>[2x]MKVQYSFEREFEELMSDLLSKYGYEMFQMDGLGDQLDVVKFTEDFVRRGIIESTIDANANVRVTNISTYFIEISKPHTYLYSLYRIWQKMKEMFGKGVADEFVEAQINGAVYLHDRHHAALMPYCFAYTLKPIVEKGLPFIKTIKSEPAKHLSTFIQHVIQFVMFASNQSSGAVGLPDFFVWMWYFVKKDLKEGIIPRDKLDWYIEQHFQILTYSLNQPIRTTQSPYTNFTYLDRNYIKAIFEGERYPDGSLITDHVEDIIALQKHYWEWVSRERERQMFTFPVLTASLLYKDGKFLDEDSARFINKINMKWQDTNWYISDSIDAVASCCRLTSSTQTLKKFSLSSEEEEKLKGRMNSIGGSDLNIGSFKVITVNLPRIALESGGDREKYLQILRHRVQLIKKALAAVREIIKERISEGLLPLYENGLMLLNRQYGTIGVTGVWESASIMGLTTEDIDGLKYTEEGEVFVDNVLDTIREEAEKGYHEYGFTFNIEQVPAEKAAVTLAQKDRFLFGEKQPFEIYSNQWVPLMANTDVLNRIRYSGKWDKKVSGGAILHINLGESFKTEEESFNMVKMIADMGVMYFAFNTKISVCEDGHAFYGERCPVCGKAKVDEYMRIVGYLVPVSAFNKERREIEYPRRQFYDSLTIRR

Ribonucleotide reductases (RNRs) are highly important enzymes for all life, as they are solely responsible for the first committed step in the synthesis of the deoxyribonucleoside triphosphate (dNTP) building blocks of DNA. Class III RNRs, strictly anaerobic, generate on a separate activating enzyme NrdG the same type of 5’-dAdo radical through homolytic cleavage of a C-S bond in S-adenosylmethionine, with the participation of a [4Fe-4S] cluster. Here we present the crystal structure of a second class III RNR from Thermotoga maritima (tmNrdD), which, as purified and crystallized, surprisingly does not display such a cysteine, possessing an isoleucine (Ile) in its place. Nevertheless tmNrdD binds a substrate and its allosteric effector in productive conformations as expected from previous structures of RNRs of all three classes, and it is enzymatically active.

The native structure was solved from crystals obtained under three different conditions, one with the buffer molecule citrate bound in the active site, another with MES and a third with glycerol. S1 Fig Occupancy of the active site of tmNrdD by various buffer components. As in T4NrdD, the α-β barrel is decorated by an extra Zn-ribbon domain inserted between the last strand of the barrel and the C-terminal loop containing the glycyl radical site. The identity of the metal ion has been confirmed by anomalous diffraction at the Zn and Fe K edges. The Zn2+ ion is coordinated by the motif CxxxHx6CxxC [CxxCx14CxxC in the T4 and E. coli enzymes]. The tmNrdD structure contains a C-terminal loop harbouring the glycyl radical site (Gly621), which dips into the α-β barrel such that its tip meets that of the finger loop in the active site. Since the T4 enzyme structure was solved as an oxygen-insensitive Gly->Ala mutant, the present structure allows the native conformation of the radical Gly in an anaerobic ribonucleotide reductase to be observed in its resting state prior to activation, as also seen by Wei et al.. Gly621 itself is completely buried from solvent and presumably undergoes a significant conformational change in order for its hydrogen atom to be abstracted by the 5’-dAdo radical generated by the activase, as postulated previously for T4NrdD and PFL.>SNAMKTQVAIIGAGPSGLLLGQLLHKAGIDNIIVERQTAEYVLGRIRAGVLEQGTVDLLREAGVAERMDREGLVHEGVELLVGGRRQRLDLKALTGGKTVMVYGQTEVTRDLMQAREASGAPIIYSAANVQPHELKGEKPYLTFEKDGRVQRIDCDYIAGCDGFHGISRQSIPEGVLKQYERVYPFGWLGLLSDTPPVNHELIYAHHERGFALCSQRSQTRSRYYLQVPLQDRVEEWSDERFWDELKARLPAEVAADLVTGPALEKSIAPLRSLVVEPMQYGHLFLVGDAAHIVPPTGAKGLNLAASDVNYLYRILVKVYHEGRVDLLAQYSPLALRRVWKGERFSWFMTQLLHDFGSHKDAWDQKMQEADREYFLTSPAGLVNIAE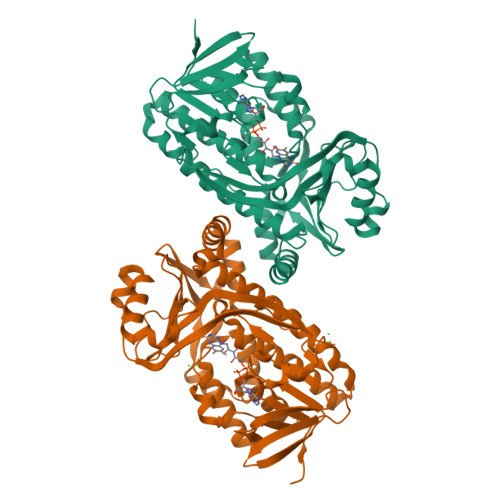NYVGLPFEEVA[4x]> MSFTLIQQATPRLHRSELAVPGSNPTFMEKSAASKADVIFLDLEDAVAPDDKEQARKNIIQALNDLDWGNKTMMIRINGLDTHYMYRDVVDIVEACPRLDMILIPKVGVPADVYAIDVLTTQIEQAKKREKKIGFEVLIETALGMANVEAIATSSKRLEAMSFGVADYAASTRARSTVIGGVNADYSVLTDKDEAGNRQTHWQDPWLFAQNRMLVACRAYGLRPIDGPFGDFSDPDGYTSAARRCAALGFEGKWAIHPSQIDLANEVFTPSEAEVTKARRILEAMEEAAKAGRGAVSLDGRLIDIASIRMAEALIQKADAMGGKE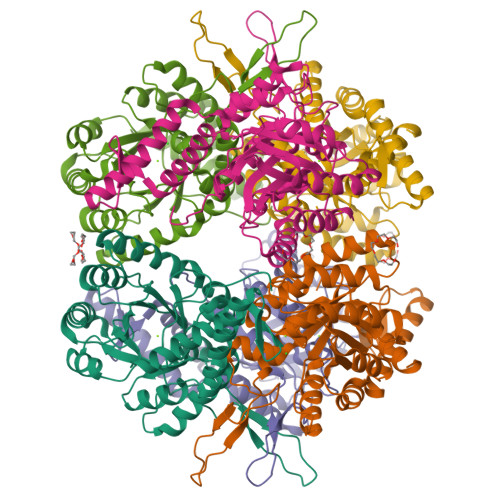HHHHHHHH> MGEVKSVKVDNWGVFFLQKLQNFFNKTDYCDLTLQFRDNSQLKVHRLVLSACTDYFNVLEQTCEIVDDALIMPNEFQADVVVPIVNFMYTGTLEFELKMYGKLLRTAKEMNMTVLLKLLEAHRRTMENVNRQQRHHHHHH

Particularly, Centrosomal Protein 190 (CP190), a protein originally described for its ability to bind to the centrosome during mitosis, was shown to play a crucial role in the insulation function of various IBPs. CP190 is composed of a BTB (bric-a-brac, tramrack, and broad complex)/POZ (poxvirus and zinc-finger) domain, four predicted C2H2 zinc-finger motifs, and an E-rich, C-terminal region. We propose a general model for insulator function in which BEAF32/dCTCF/Su(HW) provide DNA specificity (first layer proteins) whereas CP190/Chromator are responsible for the physical interactions required for long-range contacts (second layer). BTB/POZ are a family of protein-protein interaction motifs conserved from Drosophila to mammals, and present in a variety of transcriptional regulators.

Overall, the FCCS data strongly suggest that the BTB/POZ domain of CP190 is involved in the direct protein-protein interactions required for the establishment of long-range contacts. To directly test this hypothesis, we solved the crystal structure of the CP190-BTB/POZ. The CP190-BTB/POZ domain crystallized as a stable and symmetric homodimer, in agreement with gel-filtration analysis. The overall structure is similar to classic BTB/POZ-ZF transcriptional factors where the N-terminal BTB/POZ domain is followed by several Zinc-Fingers domains. The dimerization interface is stabilized by a swapped β-strand that forms a long groove where extended polypeptidic segments can bind in order to recruit other protein partners. The dimer interface (1902 Å2/monomer according to PISA 1.47) is composed of numerous hydrophobic interactions mainly from alpha helices α1 and α2 (i.e. W12, F15, F16, F23, L47…). The native homodimeric organization is also reinforced by the N-terminal strand (residues Glu2 to Asp10) being swapped: the β1 stand of a monomer interacts with the β5 strand of the other monomer. The sequence conservation among CP190 orthologs from insects (55 sequences analyzed using CONSURF) show little conservation besides the domain core, the dimerization interface and the peptide binding groove. Interestingly, this suggests that CP190-BTB/POZ does not form higher order macromolecular assemblies by itself while partner recruitment requires homo-dimerization. Here, we showed that the BTB/POZ domains of CP190 forms homo-dimers with a large, conserved interaction surface, consistent with these domains being responsible for the formation of the direct protein-protein interactions required for the establishment of long-range contacts.> SAQDKLIKPSHLITMDDIIREGNPTLRAVAKEVSLPLCDEDILLGEKMMQFLKHSQDPVMAEKLGLRAGVGLAAPQIDVSKRIIAVLVPNLPDKEGNPPKEAYSWQEVLYNPKIVSHSVQDAALSDGEGCLSVDRVVEGY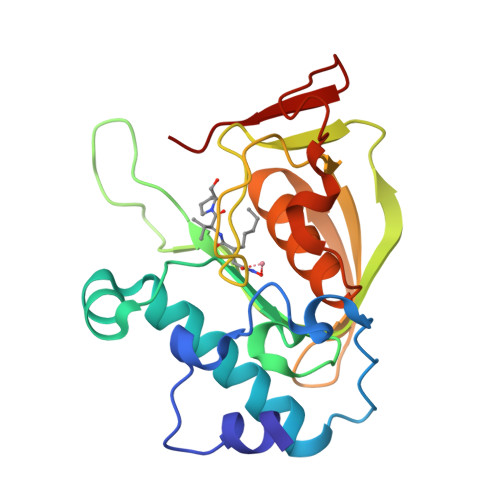VVRHARVTVDYYDKEGQQHRIKLKGYNAIVVQHEIDHINGVLFYDRINAKNPFETKEELLILDLE>[2x]GSMAQQMAFDISVNASKTINALVYFSTQQNKLVIRNEVNDTHYTVEFDRDKVVDTFISYNRHNDTIEIRGVLPEETNIGCAVNTPVSMT

The vaccinia virus protein A46 is one of a series of proteins preventing expression of host proteins that induce an anti-viral state. The A46 protein acts close to the plasma membrane by binding numerous TIR-domain containing adaptor proteins such as MyD88, MAL/TIRAP, TRAM and TRIF as well as TLR4 to prohibit further signal propagation. The VACV intracellular immunomodulators form a family of Bcl-2-like (B-cell lymphoma 2 like) proteins with low sequence identity but high structural similarity to the eukaryotic Bcl-2 protein family. Here, we report the crystal structure of the A46 N-terminal domain comprising residues 1 to 76 and demonstrate that this domain binds fatty acids.

A46(1–83) crystallized with two molecules in the asymmetric unit; electron density for a bound ligand, later identified as myristic acid, was found inside one of the molecules. The two A46 molecules comprise two β-sheets arranged head to head as an extended β-sandwich. A tetramer is formed over a crystallographic twofold axis continuing the β-sandwich with the second dimer rotated approximately 90° relative to the first. The A and B independent subunits show marked differences, with a Cα rmsd of 1.3 Å for the 45 common β-strand residues; the tetramer can be described as an A/B/B/A arrangement. Subunit A has 7 β-strands whereas subunit B presents only 6, lacking the most C-terminal one. No electron density is seen for either residues 77–83 in subunit A or 67–83 in subunit B, suggesting that these regions may constitute a flexible linker between N- and C-terminal domains in the full-length molecule. A striking feature of the external β1-β7 face of the A subunit is a partially hydrophobic tunnel, spanning the whole subunit A and reaching into subunit B. In the X-ray structure of A46(1–83), clear electron density for C14:0 myristic acid was found, with the hydrophobic tail buried in the cavity whereas the carboxyl group is open to the solvent. Tyr37 adopts a dual conformation in the two subunits, suggesting a gate-keeper role as it folds back in subunit A to make room for the myristic acid. An acceptable alternative hypothesis would be that the bound fatty acids induce asymmetry of the A46(1–83) dimer, as they block a polymerization interface equivalent to B/B and prevent binding of a second fatty acid copy in subunit B. In such manner, using the same primary sequence, a dimer of heterodimers is formed that allows utilization of different interfaces for distinct functions such as tetramerization (interface B with 6 β-strands only) or binding of cellular targets (interface A with 7 β-strands).>[2x]GAMDPDLEATLRAIVHSATSLVDARYGAMGVHDRQHRVLHFVYEGIDEETVRRIGHLPKGLGVIGLLIEDPKPLRLDDVSAHPASIGFP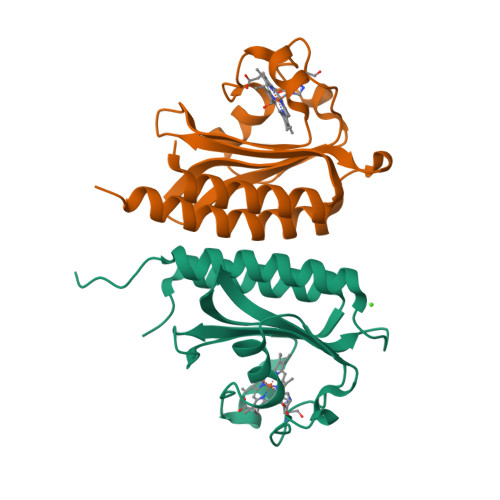PYHPPMRTFLGVPVRVRDESFGTLYLTDKTNGQPFSDDDEVLVQALAAAAGIAVANARLYQQAK>[2x]MDTNPCEKHSCIAVIDAGSTGSRLHIYSYDTDDTNTPIHIEEIWNKKIKPGFASIQPNSVTIDAYLTMLLADAPIHNIPVYFYATAGMRLLPQSQQKKYYDELDYWFRQQSQWQLVEAKTITGNDEALFDWLAVNYKLDTLKSVQ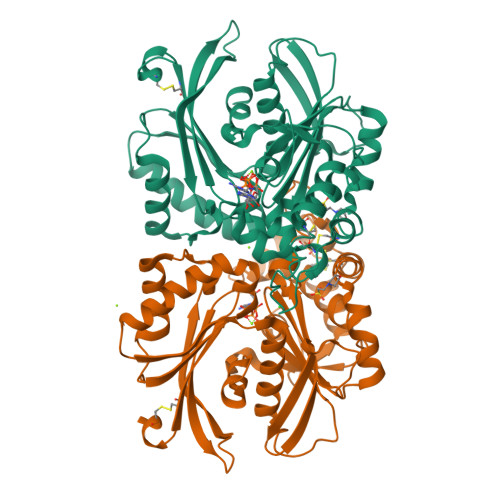NKSVGVMDMGGASVEIVFPMPKNAEISKHNQVELNIYGQNINLYVHSFLGLGQTEMSHQFLNSPSCFANDYPLPDGESGQGNAPSCKEEVTSLMNSVHKVNQQIQPLLALNPVNEWYSIGGISNLASSQLFHFENSELTNQSLLQQGDNQICHQQWDILNGQYPDDEYLYQYCLLSSYYYALMVDGYGINPNQTIHYIPPEQNLDWTIGVVLHRALEHHHHHH5-methyl-4-(methylamino)-2-(2-phenylethyl)thieno[2,3-d]pyrimidine-6-carboxylic 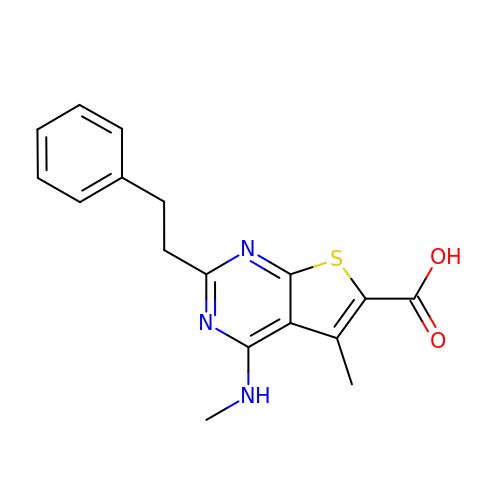acid | C17 H17 N3 O2 S | WNBAQRWHLIHMSN-UHFFFAOYSA-N>ELLPEIFRQTVEHAPIAISITDLKANILYANRAFRTITGYGSEEVLGKNESILSNGTTPRLVYQALWGR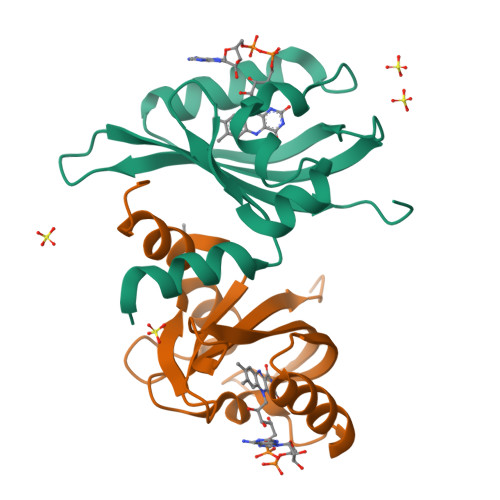LAQKKPWSGVLVNRRKDKTLYLAELTVAPVLNEAGETIYYLGMHRDTSELH[2x]Rab proteins, the biggest subfamily within the superfamily of small GTPases, are major regulators of vesicular trafficking in eukaryotic cells. One such family of effector proteins that was reported to link Rab proteins and the cytoskeleton is the Mical (molecules interacting with CasL) family. In this publication, we present a thorough biochemical and structural analysis of a Rab effector domain termed bivalent Mical/EHBP Rab binding (bMERB) domain. The results show that the domains probably constitute a Rab8-effector family involved in endosomal trafficking, and the Rab-binding specificity can be well explained from the 3-dimensional structures of complexes determined in this work.

Well diffracting crystals were found using the RBD of Mical-cL (residues 534–683) in complex with different Rab proteins (Rab1, Rab8 and Rab10). In all structures (Rab1:Mical-cL, Rab8:Mical-cL and Rab10:Mical-cL) we found one Rab protein bound to one molecule of Mical-cL, in agreement with the previous observations that all Rab proteins tested bind only one site in Mical-cL. Most interactions were visible between the Rab proteins and α-helix 3 of Mical-cL with some additional contributing residues from α-helix 2, forming extensive contacts involving residues within switch I and II of the Rab proteins. Whereas we observed KD values of 2.2–5.2 µM for Rab1 binding to the bMERB domains of Mical proteins and no detectable binding of Rab1 to the bMERB domains of EHBPs, we detected strong binding and ca. 100 nanomolar affinities for Rab8 and the different bMERB domains. Besides the specificity of bMERB domains towards the Rab8 family, another interesting observation was made in the ITC experiments comparing the stoichiometry of binding of Rab8 and the different RBDs: Whereas Rab8 bound in a 1:1 stoichiometry to Mical-cL and EHBP1, a 2:1 stoichiometry binding was observed for Mical-1, Mical-3 and EHBP1L1. In contrast to the main interacting helix α3, which adopts a similar position in all three structures, we observed slightly different orientations of the α-helices 1 and 2, adopting a position slightly further away from Rab1 compared to Rab8 and Rab10. Interestingly, whereas Rab1 contains a glutamate near the N-terminus (Glu4), all Rab8 family members contain one or (in the case of Rab10) two lysine residues in this region that point towards a negatively charged patch in Mical-cL. The sequence of the N-terminal residues of each Rab protein is shown below the corresponding structure: Whereas Rab1 contains a negatively charged glutamate at position 4, Rab8 and Rab10 contain one or two lysine residues at position 3 or at position 3 and 4, respectively. (c) Consistently, ITC measurements show that the affinity of binding increases approximately five-fold after mutating the N-terminal residues (Rab1:Mical-cL: KD = 5.2 µM; Rab1R8N:Mical-cL: KD = 1.1 µM; Rab8:Mical-cL: KD = 0.23 µM).

> GHMAKTYDYLFKLLLIGDSGVGKTCVLFRFSEDAFNSTFISTIGIDFKIRTIELDGKRIKLQIWDTAGQERFRTITTAYYRGAMGIMLVYDITNEKSFDNIRNWIRNIEEHASADVEKMILGNKCDVNDKRQVSKERGEKLALDYGIKFMETSAKANINVENAFFTLARDIKAKMDKKLEGNSPQGSNQGVKITPDQQKRSSFFRCVLL;> GHMKQEELKRLYKAQAIQRQLEEVEERQRASEIQGVRLEKALRGEADSGTQDEAQLLQEWFKLVLEKNKLMRYESELLIMAQELELEDHQSRLEQKLREKMLKEESQKDEKDLNEEQEVFTELMQVIEQRDKLVDSLEEQRIREKAEDQHFES>[6x]MEFTGDLGLGHVTIR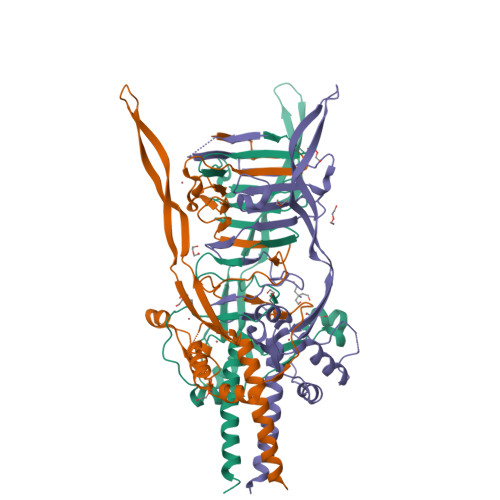ASTSSNIRSEVLMEGEYGFIGKSIPTDNPAGQRIIFCGGEGTSSTTGAQITLYGANNTDSRRIVYNGDEHLFQSADVKPYNDNVTALGGPSNRFTTAYLGSNPIVTANGERKTEPVVFDDAFLDAWGDVHYIMYQWLDAVQLKGNDARIHFGVIAQQIRDVFIAHGLMDENSTNCRYAVLCYDKYPRMTDTVFSHNEIVEHTDEEGNVTTTEEPVYTEVVIHEEGEEWGVRPDGIFFAEAAYQRRKLERIEARLSALEQK>QDMVSPPPPIADEPLTVNTGIYLIECYSLDDKAETFKVNAFLSLSWKDRRLAFDPVRSGVRVKTYEPEAIWIPEIRFVNVENARDADVVDISVSPDGTVQYLERFSARVLSPLDFRRYPFDSQTLHIYLIV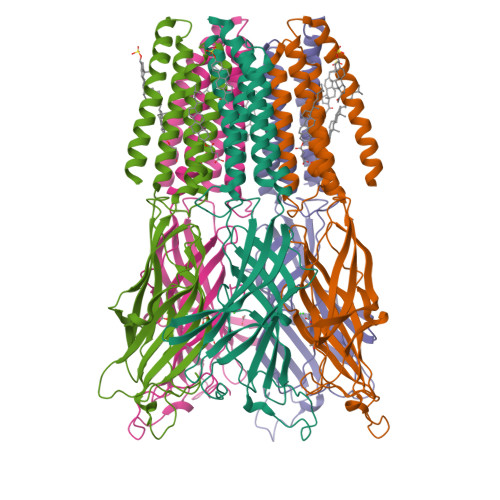RSVDTRNIVLAVDLEKVGKNDDVFLTGWDIESFTAVVKPANFALEDRLESKLDYQLRISRQYGYFVIQTYLPCIMTVILSQVSFWLNRESVPARTVFVVTTVLTMTTLSISARNSLPKVAYATAMDWFIAVCYAFVFSALIEFATVNYFTKSQPARAAKIDRLSRIAFPLLFGIFNLVYWATYLNREPQLKAPTPHQHHHHHHHH[5x]3-(1~{H}-indol-5-yl)benzoic acid | C15 H11 N O2 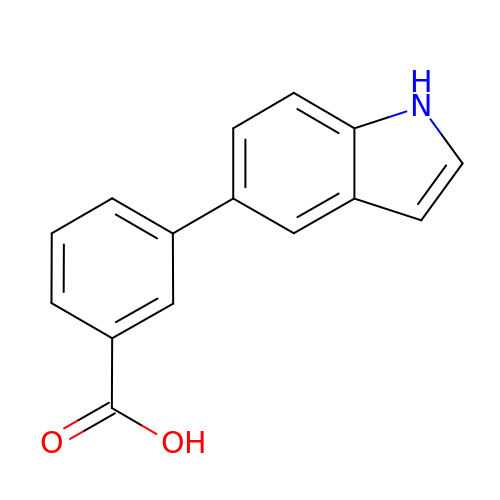| VKHHKQSCGXEKEE-UHFFFAOYSA-N> GPLGSDLKDAEAVQKFFLEEIQLGEELLAQGDYEKGVDHLTNAIAVSGQPQQLLQVLQQTLPPP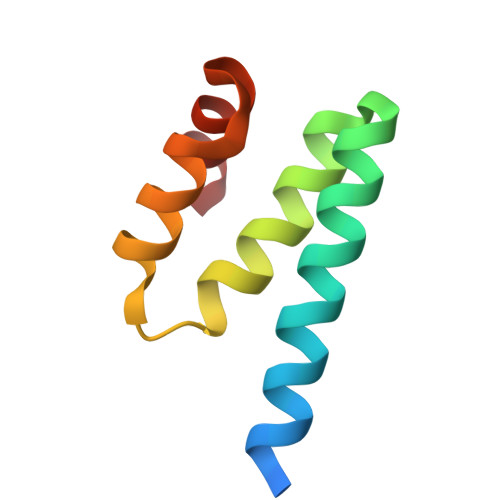VFQMLLTKL> UCCCAGUCCACCG;> CGGUGAGA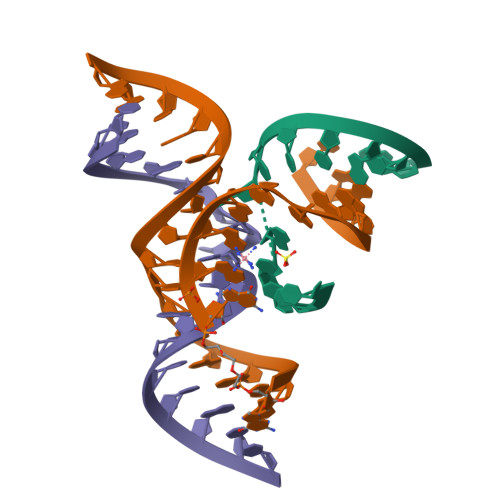AGGGXGGCAGAGAAACACACGA;> UCGUGGUGCAUUACCUGCC>GPLGSTEVLCLMNMVLPEELLDDEEYEEIVEDVRDECSKYGLVKSIEIPRPVDGVEVPGCGKIFVEFTSVFDCQKAMQGLTGRKFANRVVVTKYCDPDSYHRRDFW[2x];>[2x]GPLGSSKKRKRSRWNQDTMEQKTVIPGMPTVIPPGLTREQERAYIVQLQIEDLTRKLRTGDLGIPPNPEDRSPS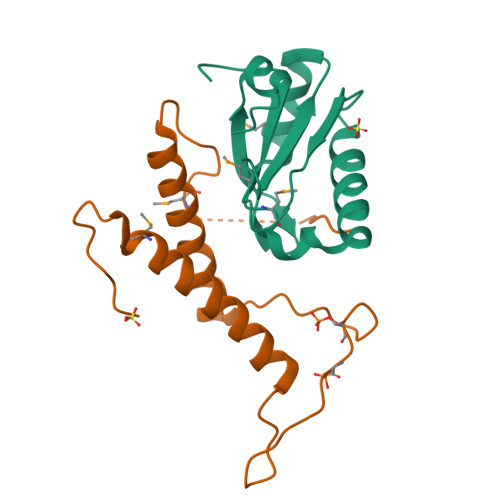PEPIYNSEGKRLNTREFRTRKKLEEERHNLITEMVALNPDFKPPADYKPP> AVTKLVLVRHGESQWNKENRFTGWYDVDLSEKGVSEAKAAGKLLKEEGYSFDFAYTSVLKRAIHTLWNVLDELDQAWLPVEKSWKLNERHYGALQGLNKAETAEKYGDEQVKQWRRGFAVTPPELTKDDERYPGHDPRYAKLSEKELPLT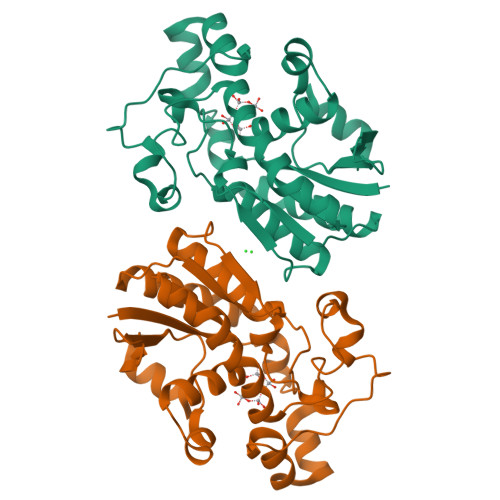ESLALTIDRVIPYWNETILPRMKSGERVIIAAHGNSLRALVKYLDNMSEEEILELNIPTGVPLVYEFDENFKPLKRYYLGNADEIAAKAAAVANQGKAK> MASWSHPQFEKGAHMVRKMRIAVIDYDKCNPDKCGHFLCERVCPVNRMGGEAIIIDEENYKPIIQEASCTGCGICVHKCPFNAISIVNLPEQLDEDCVHRYGVNAFVLYRLPIVKDGMVVGIVGPNGTGKTTAVKILAGQLIPNLCEDNDSWDNVIRAFRGNELQNYFERLKNGEIRPVVKPQYVDLLPKAVKGKVRELLKKVDEVGKFEEVVKELEL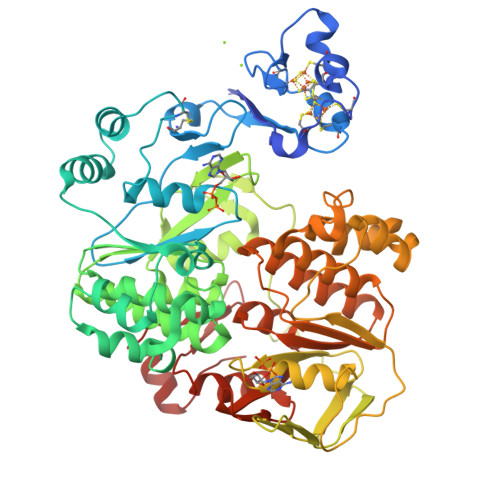ENVLDRELHQLSGGELQRVAIAAALLRKAHFYFFDEPSSYLDIRQRLKVARVIRRLANEGKAVLVVEHDLAVLDYLSDVIHVVYGEPGVYGIFSKPKGTRNGINEFLQGYLKDENVRFRPYEIRFTKLSERVDVERETLVEYPRLVKDYGSFKLEVEPGEIRKGEVIGIVGPNGIGKTTFVKMLAGVEEPTEGKVEWDLTVAYKPQYIKAEYEGTVYELLSKIDSSKLNSNFYKTELLKPLGIIDLYDRNVEDLSGGELQRVAIAATLLRDADIYLLDEPSAYLDVEQRLAVSRAIRHLMEKNEKTALVVEHDVLMIDYVSDRLIVFEGEPGRHGRALPPMGMREGMNRFLASVGITFRRDPDSGRPRANKEGSVKDREQKARGEYYYA> GSENIYTTLKFESMMQQRVIQIRSIPEEEYHELVSVQFKTDGGKYEKGEKQDLELSEKKTENGKDTESWGWNENQDSDEHDGWDEELDIDVDNVPIQVSVFVQSAAKVFTEFEQGCDTIGRSKVESIYLYKFNLLQTAFFAMVSEKVNDWTQLYKDVRYLYTENPKLLQLMELNSRRLDLNLNLIKKTIYKLVNDQLQELKDNERTPDWDITISSLLPYLKKTALPTLYKLEDNTILVALIRYIVHDLVIDNILHWRVISEKSSENLSEFIMLLLSGLEIPRLNLIETYRHSREKLGILSKILTAHLKDILEMFYEGEFFLFETDEIVQWIILLFADTPTRRDCIDEIRRVREEATD;> MLEEQLYLLACIFASRA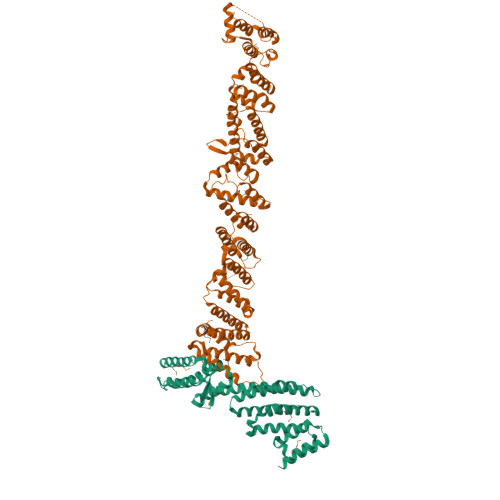DTRNIKKLSTRLGSQSKYLEILCVLWPELDDPKNLLFLRELEEEVQSPEGEETTDEDVIVELLESDSSLIPLIESDTTTRSNRYHELQEFISKKLNNKTLENFEEWLRERILICNEMIPETPLLYSVLWETAKSKVLSTKFIGWVEGVLKPLDHLNKRLHLIFKINEWEKMPDSELFKIIFDGVEDMQGYIGIADVIEDELAPTLSYGKKWETFITEFFNKQQFSLKSDTNYQLFIKLYYSLEKGVKDNSEASRKLQSNVVDILFHNSENLFNLSSLTHKLDELWSILSGFPDEITIEEQKTITALEMKQFMEFFIKCSTKFSFKEIFAITQEEESAQLAHFSSLCHEEFNKANEISSFLQAMYETVLDISKDDKIFTRISMDEKLYSILEILLQMNEFAYIEAIIERFDYSNNTQIYELLVKFFWHFFNNASNGLRKEPEMKKASQTLQIIQKHMSQRAGTNLTKLEVLLEISDKLSHYSINLNKSHNGARDTAFKPSNILEYRDCPLDIISNLLELNPRLYKDLPTTKSLLFGIYDSLSINREGQTGKVEVDLMVLHIDYALVNLDFGTAYELGKQVFEICQEAGQHMMKALGDEHWLTFYQMGKFVDPNWVDNEIPTEIIVLQMSILGRLLEVCPLEEVEIVTSQWSTLELELSARDLVKDKYALDGQNDNKSKVGGIAREIFHNVTNF> PGEWAGKDKIEKVSIYMVPQGGPGLVESAEDLDFGTYYENPTIDPATHNAILKPKKGIKVNSAVGKTVKVYVVLNDIAGKAKALLANVNAADFDAKFKEIIELSTQAQALGTVADGPNPATAAGKIAKKNGTTDETIMMTCLQPSDALTIEEAAVSEANAIAGIKNQAKVTVERSVARAMVSTKAQSYEIKATTQIGEIAAGSVLATITDIRWVVAQGERRQYLSKKRGTVPENTWVTPGSGFVPTSSTFHTNATEYYDYAGLWEDHNTNEAVISGTQVPTLADYQLQDVTGELANALSGKFLLPNTHKSGANAASSDYKRGNTAYVLVRAKFTPKKEAFIDRGKTYSDNTAVPEYVAGEDFFVGENGQFYVSMKSVTDPKVGGVAGMKAHKYVKGKVLYYAWLNPSTTSPDSWWNSPVVRNNIYHIHIKSIKKLGFNWNPLVPDPDPSNPENPNNPDPNPDEPGTPVPTDPENPLPDQDTFMSVEVTVLPWKVHSYEVDL

P. gingivalis displays two forms of fimbriae on its surface, FimA and Mfa1, both of which are crucial for attachment to other bacteria in the oral biofilm and to the host cells. In the work presented herein we have determined the crystal structures of the shaft protein Mfa1, in both mature and precursor forms, the anchor protein Mfa2 and a truncated precursor form of the tip protein, Mfa3. The resulting mature protein thereby has an empty position in the first β-sheet that a β-strand donated from another fimbrial protein presumably fills in order to polymerize the individual proteins into a polymeric fimbria.

Instead, the mature form, mMfa1, which could be purified as a monomer, was used for crystallization and structure determination. The mMfa1 structure revealed that its C-terminus was partly located in the position where the N-terminal extension is expected to be embedded, based on previous structural studies of related proteins. Further, the C-domain consists of a mixture of β-strands, β-hairpins, coils and a few short helices. mMfa1 has the same overall structure as pMfa1Δ9 but, as a consequence of the missing β1-strand, a void is formed in sheet 1 which is partly filled by the final C-terminal residues. The absence of the β1-strand in mMfa1 induces some disorder in the N-domain; there is no interpretable density for residues 215–229 (a short helix and a coiled region). In mMfa1, the long C-terminus fills the same position as β1 does in the precursor form, albeit running in the opposite direction. Tyr559, Val561 and Leu563 fill the hydrophobic pockets that otherwise hold Met43, Leu41 and Met39. The C-terminus does not reach through the whole sheet, leaving the short helix, described above, and part of the neighbouring strand disordered. The protein binds one metal ion, modelled as Ca2+ due to the high concentration of Ca2+ ions in the crystallization buffer. The metal ion is coordinated by the side chain oxygens of Asp507 (bidentate), Asp509 (monodentate), and Asn512 and the main chain carbonyl oxygens of Asp207, Asn512, and Gln514. Instead, the end of the C-terminus reaches to its own empty β1-position and partially fills it.>MSQLVECVPNFSEGNNQEVIDAISQAISQTPGCVLLDVDAGPSTNRTVYTFVGQPECVVEGALSAARTASQLIDMRKHKGEHPRMGALDVCPFIPVRGVSMDECVLCAKAFGQRLAEELNVPVYLYGEAAQMPSRQTLPAIRAGEYEALPEKLKQAEWVPDFGPSSFVPSWGATVTGARKFLIAFNINLLSTKEQAHRIALNLREQGRGKDQPGRLKKVQGIGWYLEEKNLAQVSTNLLDFEVTALHTVYEEARREAQELNLPVVGSQLVGLVPLKALLDAAAFYCDKEKLFVLEEEHRIRLVVNRLGLDSLAPFDPKERIIEYLVPDSGPEQSLLDASLRAFVREVGARSAAPGGGSVAAAVAALGAALASMVGQMTYGRRQF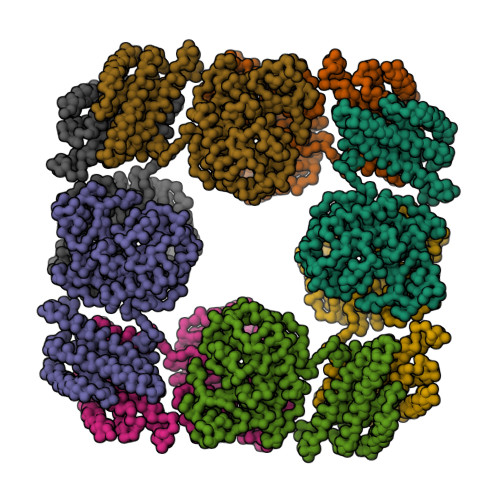DHLDSTMRRLIPPFHAASAQLTSLVDADARAFAACLGAIKLPKNTPEERDRRTCALQEGLRQAVAVPLKLAETVSQLWPALQELAQCGNLSCLSDLQVAAKALETGVFGAYFNVLINLKDMTDDVFKEKTRHRISSLLQEAKTQAALVLGSLEARKE[4x]>VLDGPYQPTRFKPPNDYWILLSPTNQQVVLEGTNRTDVWVALLLVEPNVTNQSRQYTLFGETKQITVENNTNKWKFYEMFRNSASAEFQHKRTLTSDTKLAGFLKHGGRVWTFYGETPHATTDYSSTSNLSEVETVIRTEFYIIPRSQESKCN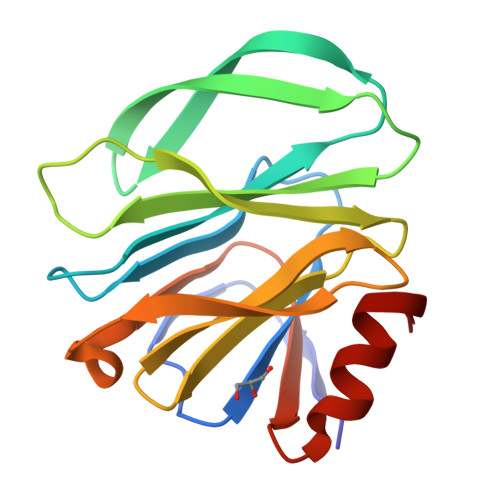EYINTGL[4x]> SSLDDKPQFPGASAEFIDKLEFIQPNVISGIPIYRVMDRQGQIINPSEDPHLPKEKVLKLYKSMTLLNTMDRILYESQRQGRISFYMTNYGEEGTHVGSAAALDNTDLVFGQYREAGVLMYRDYPLELFMAQCYGNISDLGKGRQMPVHYGCKERHFVTISSPLATQIPQAVGAAYAAKRANANR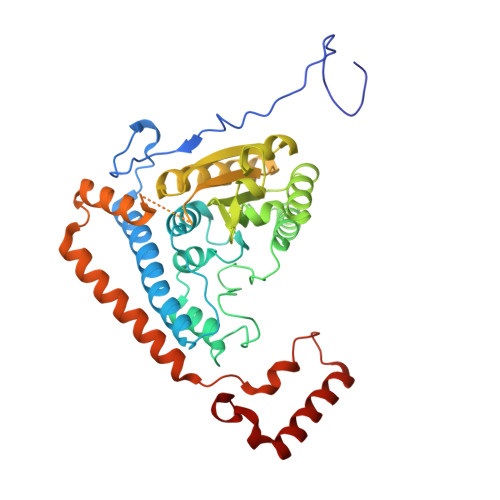VVICYFGEGAASEGDAHAGFNFAATLECPIIFFCRNNGYAISTPTSEQYRGDGIAARGPGYGIMSIRVDGNDVFAVYNATKEARRRAVAENQPFLIEAMTYRIGHHNTSDDSSAYRSVDEVNYWDKQDHPISRLRHYLLSQGWWDEEQEKAWRKQSRRKVMEAFEQAERKPKPNPNLLFSDVYQEMPAQLRKQQESLARHLQTYGEHYPLDHFDK>GSHMASMTGGQQMGRGSMISVLFVCLGNICRSPMAEAIFRDLAAKKGLEGKIKADSAGIGGWHIGNPPHEGTQEILRREGISFDGMLARQVSEQDLDDFDYIIAMDAENIGSLRSMAGFKNTSHIKRLLD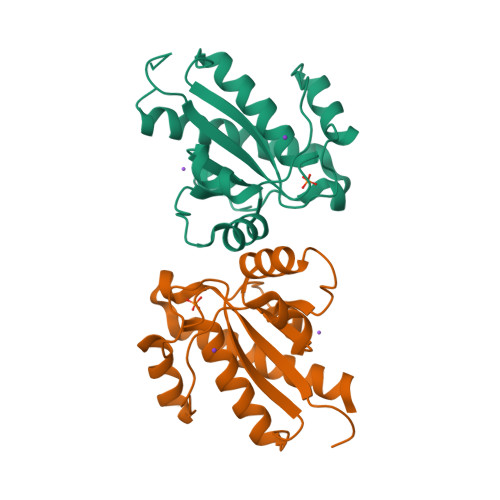YVEDSDLADVPDPYYTGNFEEVCQLIKTGCEQLLASIQKEKQL[2x]> AQTVPYGIPLIKADKVQAQGFKGANVKVAVLDTGIQASHPDLNVVGGASFVAGEAYNTDGNGHGTHVAGTVAALDNTTGVLGVAPSVSLYAVKVLNSSGSGSYSGIVSGIEWATTNGMDVINMSLGGASGSTAMKQAVDNAYARGVVVVAAAGNSGNSGSTNTIGYPAKYDSVIAVGAVDSNSNRASFSSVGAELEVMAPGAGVYSTYPTNTYATLNGTXMASPHVAGAAA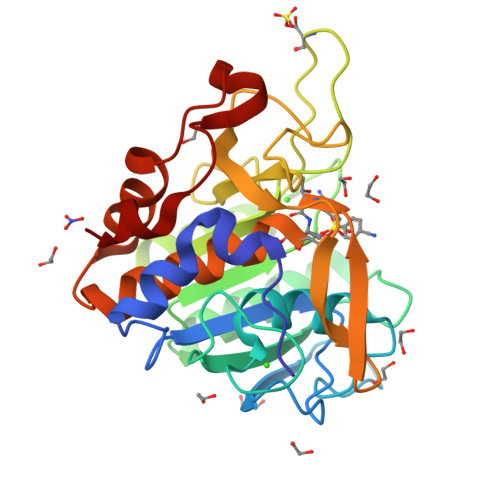LILSKHPNLSASQVRNRLSSTATYLGSSFYYGKGLINVEAAAQ> GSHMERPESELIRQSWRVVSRSPLEHGTVLFARLFALEPSLLPLFQYNG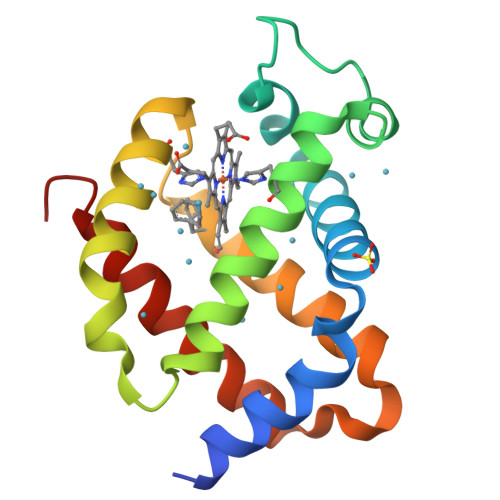RQFSSPEDSLSSPEFLDHIRKVMLVIDAAVTNVEDLSSLEEYLTSLGRKHRAVGVRLSSFSTVGESLLYMLEKSLGPDFTPATRTAWSRLYGAVVQAMSRGWDGE>[6x]MRGSHHHHHHGSMDKNIIIGAMTALITPFKNGKVDEQSYARLIKRQIENGIDAVVPVGTTGESATLTHEEARTCIEIAVETCKGTKVKVLAGA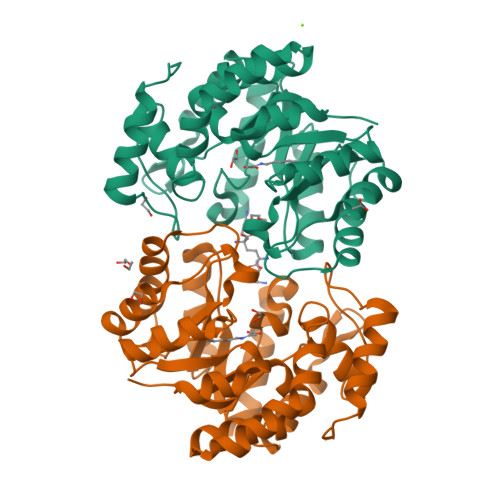GSNATHEAVGLAKFAKEHGADGILSVAPYYNKPTQQGLYEHYKAIAQSVDIPVLLYNVPGRTGCEISTDTIIKLFRDCENIYGVKEASGNIDKCVDLLAHEPRMMLISGEDAINYPILSNGGKGVISVTSNLLPDMISALTHFALDENYKEAKKINDELYNINKILFCESNPIPIKTAMYLAGLIESLEFRLPLCSPSKENFAKIEEVMKKYKIKGF> MQQTTQIQPSFTLKTREGGVASADERADEVVIGVGPAFDKHQHHTLIDMPHGAILKELIAGVEEEGLHARVVRILRTSDVSFMAWDAANLSGSGIGIGIQSKGTTVIHQRD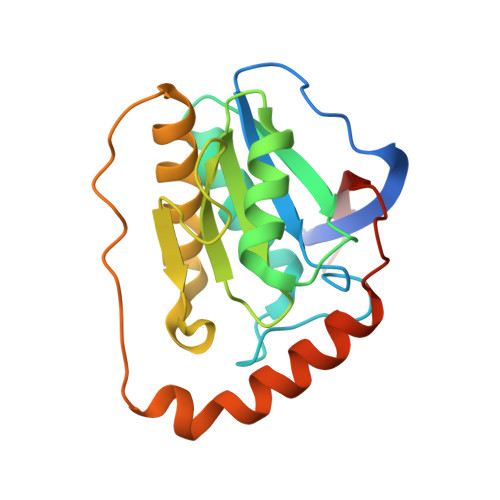LLPLSNLELFSQAPLLTLETYRQIGKNAARYARKESPSPVPVVNDQMVRPKFMAKAALFHIKETKHVVQDAEPVTLHIDLVRE> MEDPLIGRDSLGGGGTDRVRRSEAITHGTPFQKAAALVDLAEDGIGLPVEILDQSSFGESARYYFIFTRLDLIWSLNYFALLFLNFFEQPLWCEKNPKPSCKDRDYYYLGELPYLTNAESIIYEVITLAILLVHTFFPISYEGSRIFWTSRLNLVKVACVVILFVDVLVDFLYLSPLAFDFLPFRIAPYVRVIIFILSIRELRDTLVLLSGMLGTYLNILALWMLFLLFASWIAFVMFEDTQQGLTVFTSYGATLYQMFILFTTSNNPDVWIPAYKSSRWSSVFFVLYVLIGVYFVTNLILAVVYDSFKEQLAKQVSGMDQMKRRMLEKAFGLIDSDKNGEIDKNQCIKLFEQLTNYRTLPKISKEEFGLIFDELDDTRDFKINKDEFADLCQAIALRFQKEEVPSLFEHFPQIYHSALSQQLRAFVRSPNFGYAISFILIINFIAVVVETTLDIEESSAQKPWQVAEFVFGWIYVLEMALKIYTYGFENYWREGANRFDFL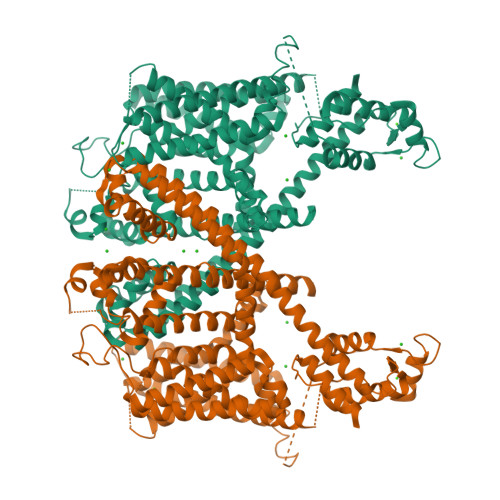VTWVIVIGETATFITPDENTFFSNGEWIRYLLLARMLRLIRLLMNVQRYRAFIATFITLIPSLMPYLGTIFCVLCIYCSIGVQVFGGLVNAGNKKLFETELAEDDYLLFNFNDYPNGMVTLFNLLVMGNWQVWMESYKDLTGTWWSITYFVSFYVITILLLLNLVVAFVLEAFFTELDLEEEEKCQGQDSQEKRNRRRSAGSKSRSQRVDTLLHHMLGDELSKPECSTSDTSTAGLVPR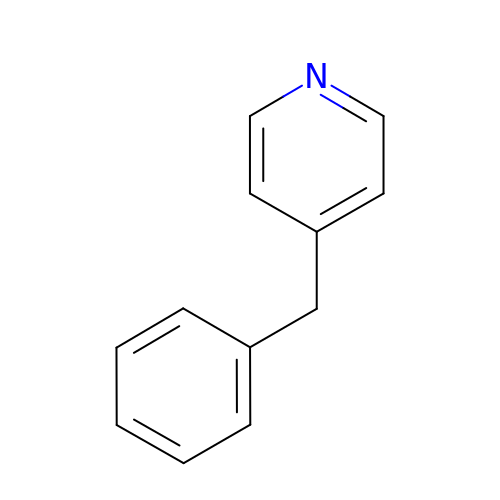4-benzylpyridine | C12 H11 N | DBOLXXRVIFGDTI-UHFFFAOYSA-N> GHMLFISATNTNAGKTTCARLLAQYCNACGVKTILLKPIETGVNDAINHSSDAHLFLQDNRLL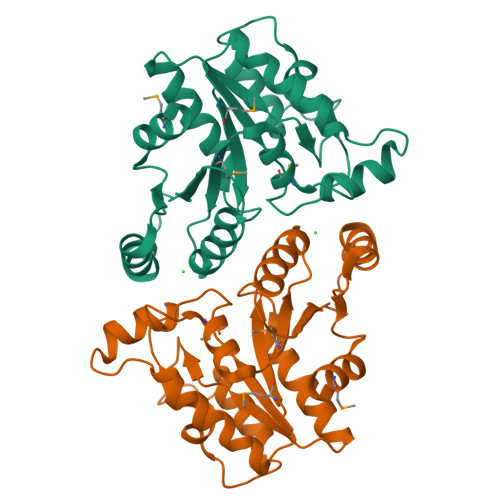DRSLTLKDISFYRYHKVSAPLIAQQEEDPNAPIDTDNLTQRLHNFTKTYDLVIVEGAGGLCVPITLEENMLDFALKLKAKMLLISHDNLGLINDCLLNDFLLKSHQLDYKIAINLKGNNTAFHSISLPYIELFNTRSNNPIVIFQQSLKVLMSFALK>MEPVKCNLCYECIESDELRANCPFTDCNSINHLTCLASSFLTEE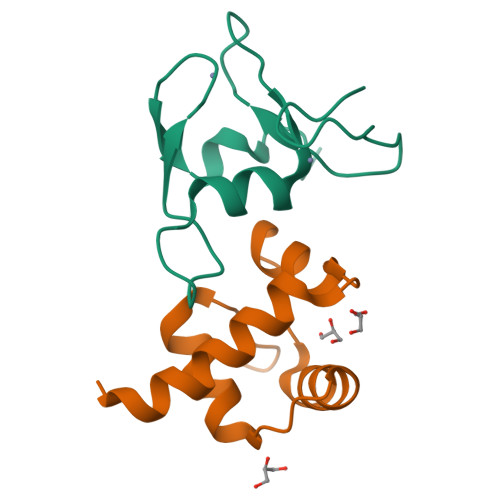CQVLPIEGMCTKCKRVLRWREFLSTVFTT[2x];>[2x]GSMIVTQTHRAISQVVKQAKDNSVWIKILTYSAIDVEEFQLWLKRKNLNVSLDLIKSWCDKYGVLMKGSWH> MPLVKRNIDPRHLCHTALPRGIKNELECVTNISLANIIRQLSSLSKYAEDIFGELFNEAHSFSFRVNSLQERVDRLSVSVTQLDPKEEELSLQDITMRKAFRSSTIQDQQLFDRKTLPIPLQETYDVCEQPPPLNILTPYRDDGKEGLKFYTNPSYFFDLWKEKMLQDTEDKRKEKRKQKQKNLDRPHEPEKVPRAPHDRRREWQKLAQGPELAEDDANLLHKHIEVANGGG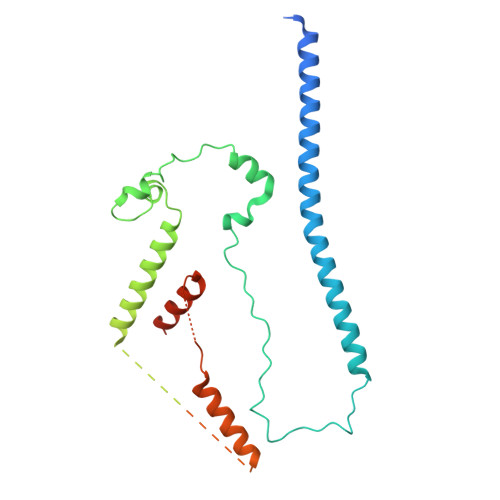SGGSGGSGGSGGSGGSKRHPSTLPVISDARSVLLEAIRKGIQLRKVEEQREQEAKHERIENDVATILSRRIAVEYSDSEDDSEFDEVDWLE Mitochondrial poration by pore-forming BCL-2 Effectors, BAK and BAX, initiates apoptosis. BAK is dormant in healthy cells. Its apo structure exhibits a stable globular conformation incapable of executing poration. Autoactivation is mechanistically similar to direct activation: binding of exposed BH3 of BAK or activators to the activation groove induces conformational changes in the electrostatic network at the bottom of this groove destabilizing helix α1 to initiate BAK unfolding.

To stabilize and structurally characterize directly activated BAK complexes, we rationally designed BID-like BH3 peptides that bind BAK with high affinity compared to WT BID BH3. Based on activity and binding profiles of monosubstituted peptides, we produced disubstituted M(3)W(5) BID-like BH3 peptide, which exhibits ~30-fold higher binding affinity for BAK compared to WT BID BH3, judged by ITC and SPR. In liposome permeabilization assays this peptide is similarly potent as WT BID BH3 in direct BAK activation according to AUC against peptide dose EC50 analysis. To reveal the structural basis of direct BAK activation we determined the crystal structure of activated covalent complex M(3)W(5) BID BH3GGC-G184C tevBAK [M(3)W(5) BID BH3-BAK] disulfide tethered as BAK BH3-BAK complex. We observed two similar complexes in the asymmetric unit, and both exhibit destabilized helix α1 electrostatic network in the protein core as observed in the BAK BH3-BAK complex (electron density shown in Supplementary Fig. 9a). Directly activated BAK exhibits 2 hydrogen bonds between α1 R42 and α2 N86. We validated BAK destabilization upon direct activation by determining Tm values of apo BAK and the M(3)W(5) BID BH3-BAK complex ± DTT. The reduced complex (15 µM, 95% peptide occupancy estimated from KD) is significantly destabilized compared to apo BAK or the covalent complex (15 µM, 100% peptide occupancy based on the crystal structure). In contrast, the cavities in activated BAK BH3-BAK and inactivated W(3)W(5) BID BH3-BAK complexes are more modest in size (64–70 Å3) whereas activated M(3)W(5) BID BH3-BAK complex exhibits no cavity at the activation groove. Our new structures (10 asymmetric unit BAK BH3-BAK complexes and 2 asymmetric unit M(3)W(5) BID BH3-BAK complexes) capture destabilization of helix α1 contacts to consolidate this mechanism as the basis of BAK activation by BH3 ligands.

>[2x]SASEEQVAQDTEEVFRSYVFYRHQQEQEAEGVAAPADPEMVTLPLQPSSTMGQVGRQLAIIGDDINRRYDSEFQTMLQHLQPTAENAYEYFTKIATSLFESGINWGRVVALLGFGYRLALHVYQHGLTGFLGQVTRFVVDFMLHHSIARWIAQRGGWVAALNLCNG;>EDIIRNIARHLAQMGDSMDRSWGGC[2x]>MNIQAIDTRHGTANQHSFSNGNCLPYTGVPFGMNFYAPQTTDQKGSWWFHPEDRTFQGYRVTHQPSPWMGDFSHLLMTPVSGSLSELSLFHAQSSYRPEESLFSPVEINLTQLRYQITSQLIPSMYGGILTIDYQQKDNHLLLTLPGRYQVKQLDDHQVAVKVINYSGCEDPDFSFYFVLHFEQPLTKWFAPSSGEDGKILLSFGNIAQQVVHFSSSFISEKQAQLNLAREISLRSTEMLQQGIADWHNYFDRLKVTHENPEHTKTFYHTLYRTFLFPQTFYELDENQQPIHYDTFSQTVRPGVLYTNNGFWDTYKTVYPLFSLIAQEKYEEMLEGFLNSYNETGFLPKWLSPDERGLMPGTLIDAVIADAAVKKIRPDLMPQFLEAMKKGATQQSERENYGRQGTLDYLKYGYVPSTYHESVNHTLDYAYSDFCISQVAKTLNDSETATFYRQQALNYQQLFNPETGFMQAKDTEGNFRPDFLDIRWGKDYAEGSAWQSSFAVYQDFAGLIKLYGSELAFEKKLIQLCNQAPNFNVEGYGFEIHEMSEMAAIDFGQLAISNQPSFHYPFLFSYIGKPEMAQPLLKQLMQTFDASPTGYPGDEDNGSMSAWYIFNSLGFYPVTPGTGEYVIGMPLVQTAEVKLSNGKQLTIQTSPNKVQQQFIHEIQLNQEKHTAPYFTHQELLNGGTLDYQLGIVPNPQNTAERPFSLSTEKLEHHHHH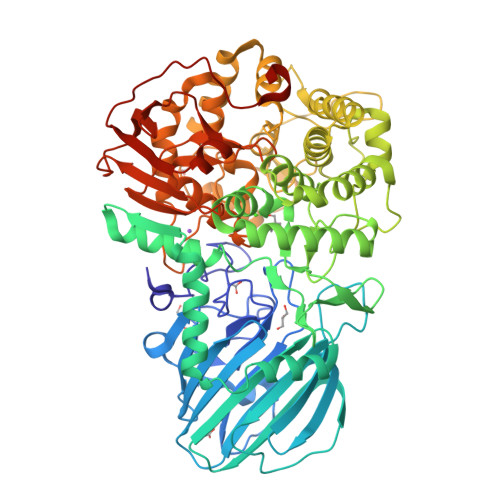H[4x]>GMAEKQYDFTHVPKRQGNSIKWGVLKEKELPMWIAEMDFKIAPEIMASMEEKLKVAAFGYESVPAEYYKAVADWEEIEHRARPKEDWCVFA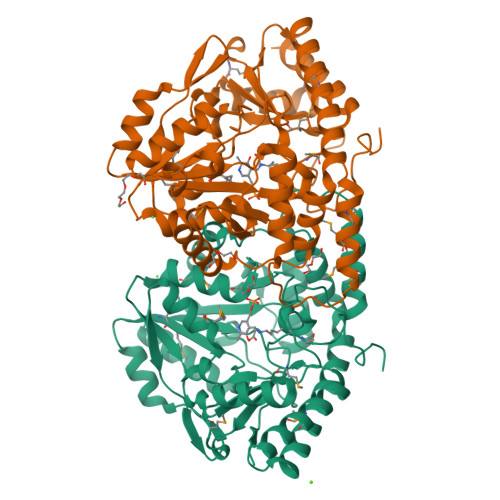SGVVPAISAMVRQFTSPGDQILVQEPVYNMFYSVIEGNGRRVISSDLIYENSKYSVNWADLEEKLATPSVRMMVFCNPHNPIGYAWSEEEVKRIAELCAKHQVLLISDEIHGDLVLTDEDITPAFTVDWDAKNWVVSLISPSKTFNLAALHAACAIIPNPDLRARAEESFFLAGIGEPNLLAIPAAIAAYEEGHDWLRELKQVLRDNFAYAREFLAKEVPEVKVLDSNASYLAWVDISALGMNAEDFCKYLREKTGLIISAGNGYRGNGHEFVRINLACPKELVIDGMQRLKQGVLNLNN[2x]Recently, Victorio and Sawyer reported the surprising, spontaneous formation of disulfide-linked dimers from a p53-derived bisthiol peptide called CV1 (CTFANLWRLLAQNC) using a mild aqueous buffer and dimethyl sulfoxide (DMSO) as oxidant. This peptide is derived from SAH-p53–8, a stapled variant of the N-terminal segment of the p53 protein that interacts with the proteins Mdm2 and MdmX. In initial studies, dimers of the CV1 peptide were determined to be exclusively antiparallel with no detectable formation of competing parallel dimers or intramolecular disulfide species. Dimerization was dependent on α-helical folding of CV1, yielding highly α-helical dimers.

Concurrent with alanine scanning and CD analyses, we also determined the three-dimensional structure of the CV1 dimer at 1.0 Å resolution. The asymmetric unit is composed of two interacting dimers. In contrast to the previously proposed dimer interface involving tryptophan residues, the structure of each dimer in the crystal structure reveals a canonical knobs-into-holes packing between Leu6, Leu9, and Leu10 as expected for a dimer of α-helices. The helical portion of each peptide is capped at the N-terminus by Thr2. Cysteine residues extend beyond the helical segment of each peptide to form bridging disulfide bonds. Asn5 and Asn13 form long-range hydrogen bonding interactions within each dimer, which is consistent with the slightly decreased stability of the N5A and N13A dimers relative to CV1 in CD experiments. For each dimer, one of the Phe3 residues and both Trp7 residues are oriented away from the dimer interface, suggesting a limited role for these residues in dimerization/disulfide bond formation. While not contributing to individual dimers, the Phe3 and Trp7 residues appear to stabilize a dimer of dimers in the asymmetric unit and help to rationalize several observations from previous and current CD data. The interface between dimers resembles a hydrophobic protein core and is composed of four copies each of Phe3, Leu6, Trp7, and Leu10. The Trp7 residues form two types of interactions: the Trp7 residues from chains B and C form a parallel displaced stacking arrangement at a distance of approximately 3.2 Å (left) while the Trp7 residues from chains A and D are parallel to each other but interacting with other hydrophobic core residues instead of each other (right).

>[4x]XCTFANLWRLLAQNCX> GGTPSPIPDPSVATVATGENGITQISSTAESFHKQNGTGTPQVETNTSEDGESSGANDSLRT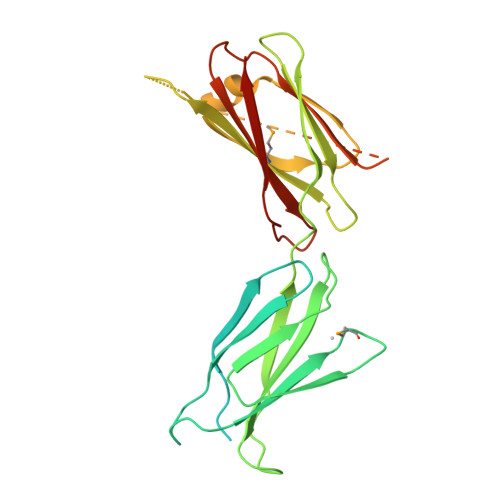PEQGSNGTDGASQKTPSSTGPSPVFDIKAVSISPTNVILTWKSNDTAASEYKYVVKHKMENEKTITVVHQPWCNITGLRPATSYVFSITPGIGNETWGDPRVIKVITEPIPVSDLRVALTGVRKAALSWSNGNGTASCRMLLESIGSHEELTQDSRLQVNISGLKPGVQYNINPYLLQSNKTKGDPLGTEGGLDASNTERSRAGSPTAPVHDESLVGPVDPSSGQQSRDTEVLLVGLEPGTRYNATVYSQAANGTEGQPQAIEFRTNAIQVFDVTA>GKKKGPKYDQIIDAAVQVIAEHGYHQAQVSKIAKAAGVADGTIYLYFNNKEDVLISLFQEKMGRFVDKIRSQMNEATDVEEKLKILVNMHFKQLAADHKLAIVTQLELRQSNTELRLKINEVLKGYLNLLDELLMEGKEKGYFFQELDTRLARQ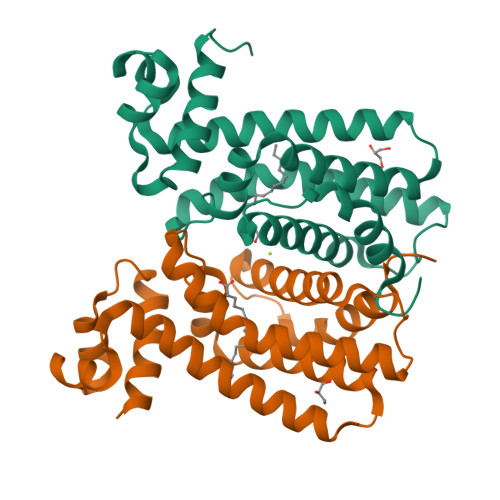MIFGTLDEVVTNWVMKDCKYDLTALVKPVHQLLLGGLRHR[2x]The mitochondrial ATP-Mg/Pi carrier (APC) is a member of the mitochondrial carrier family of transport proteins. APC is involved in the import of cytosolic adenine nucleotides into the mitochondrion and the export of inorganic phosphate from the mitochondrial matrix. Therefore, APC has the important role of altering the mitochondrial adenine nucleotide pool in order to adapt to changing cellular energetic demands. The N-terminal domain of APC forms a calcium-sensitive regulatory domain.

The consequence of calcium binding to the regulatory domain of APC is a stimulation of the substrate transport activity of the carrier. A structure of the regulatory domain of human APC isoform-1 has recently been solved, confirming the presence of four EF-hands, each of which is occupied by a bound calcium ion in a canonical pentagonal bi-pyramidal fashion. The EF-hands group together into two pairs, forming two lobes connected by a long central α-helix, in a similar fashion to the four EF-hands of calmodulin. The linker region between the N-terminal regulatory domain and the C-terminal carrier domain contains an amphipathic α-helix of unknown function. In the structure this α-helix is bound to EF-hand pair 3 and 4, analogous to the binding of a calmodulin recognition sequence motif to the hydrophobic pockets in the EF-hands of calmodulin. The protein construct used in the previous study of the HsAPC-1 regulatory domain was mutated at the extreme N-terminus to replace a cysteine residue at position 15 with a serine, raising the possibility that a native dimer could have been disrupted. Therefore, the mechanism that couples calcium binding in the regulatory domain to substrate transport in the carrier domain has not been resolved. Here, an independent structural determination of the native human APC-1 regulatory domain was completed, which was combined with an investigation into the oligomeric state of the full-length human APC-1 protein. Furthermore, an extensive comparison of the conformations of EF-hand proteins in the calcium-free, calcium-bound and peptide-bound state was undertaken, which has allowed us to propose a mechanism for the regulation of APC that is consistent with all available experimental data.

>TSEDACQDAEQPTRYETLFQALDRNGDGVVDIGELQEGLRNLGIPLGQDAEEKIFTTGDVNKDGKLDFEEFMKYLKDHEKKMKLAFKSLDKNNDGKIEASEIVQSLQTLGLTISEQQAELILQSIDVDGTMTVDWNEWRDYFLFNPVTDIEEIIRFWKHSTGIDI[3x]>MHHHHHHYQLKIEGQAPGTCGSDKSLLVSALANGIGLPYECASGGCGVCKFELLEGTVQSMWPDAPGLSSRDREKGNRHLACQCIALSDLRIKVAVQDKYIPAIPISKMEAEVVAVRALTHDLLSVKLRTDVPANFLPGQFCLIEAEQLPGVVRAYSMANSMNPDGFWEFYIKRVPTGRFSPWLFENRKVGARLFLTGPMGTSFFRPGTGRKSLCIGGGAGLSYAAAIARASIRETDKPVKLFYGSRTPRDAVRWIDIDIDEDKLEVVQAVTEDTDSLWQGPIGFIHQVVDAALLETLPEYEIYLAGPPPMVDATVRMLLGKGVPRDQIHFDAFF[3x]

Carbazole 1,9a-dioxygenase (CARDO), which consists of an oxygenase component and the electron-transport components ferredoxin (CARDO-F) and ferredoxin reductase (CARDO-R), is a Rieske nonheme iron oxygenase (RO). The electron-transport proteins of CARDO, which mediate electron transport from NAD(P)H to CARDO-O, comprise CARDO-F, which contains one Rieske-type [2Fe–2S] cluster, and CARDO-R, which contains one FAD and one plant-type [2Fe–2S] cluster. CARDO-RJ3 is a 329-residue monomeric enzyme that belongs to the FNR superfamily. It consists of three domains: an N-terminal ferredoxin (Fd) domain (residues 1–99), an FAD-binding domain (residues 100–196) and an NADH-binding domain (residues 197–329).

The type I crystals were resolved using SAD (Se atoms) and MAD (Fe atoms) experiments. The type I structure was refined at 2.6 Å resolution with a crystallo­graphic R factor of 0.249 (R free = 0.292). The type I structure contained three CARDO-RJ3 molecules per asymmetric unit; one residue (Leu289 in chain C) fell into the outlier region of the Ramachandran plot created using RAMPAGE. In both structures, electron density for one Ni2+ ion, which was deduced by analyses using the anomalous Fe-MAD map and CheckMyMetal, was observed on this axis and coordinated by two histidine residues of the N-terminal His tag from each of the three molecules. For further structural comparison we used the type I structure of CARDO-RJ3, as the FAD-bound form exhibits activity as an electron-carrier protein. The Fd domain contains a [2Fe–2S] cluster coordinated by four cysteine residues in the Cys-X 4-Cys-X 2-Cys-Xn -Cys motif. In CARDO-RJ3, Cys35, Cys40, Cys43 and Cys76 coordinate the Fe atoms of the [2Fe–2S] cluster, while the main-chain N atoms of residues 34, 36 and 38–41 form hydrogen bonds to the S atoms in the cluster. In the CARDO-RJ3 structure, the position of the main-chain O atom of Cys35 (Cys35 O) was closest to the methyl group at the C8 position (C8M) of FAD (average distance of 3.3 Å), suggesting that this orientation would be preferable for electron transfer between the two redox centres.> 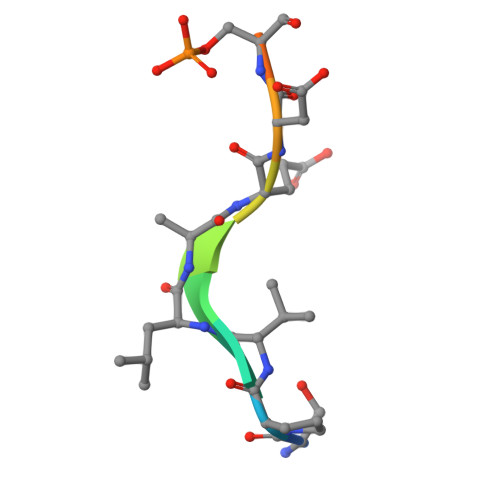SPVLAEDSEGE> MPDFLGHAENPLREEEWARLNETVIQVARRSLVGRRILDIYGPLGAGVQTVPYDEFQGVSPGAVDIVGEQETAMVFTDARKFKTIPIIYKDFLLHWRDIEAARTHNMPLDVSAAAGAAALCAQQEDELIFYGDARLGYEGLMTANGRLTVPLGDWTSPGGGFQAIVEATRKLNEQGHFGPYAVVLSPRLYSQLHRGGEIETIRQLASDGVYQSNRLRGESGVVVSTGRENMDLAVSMDMVAAYLGASRMN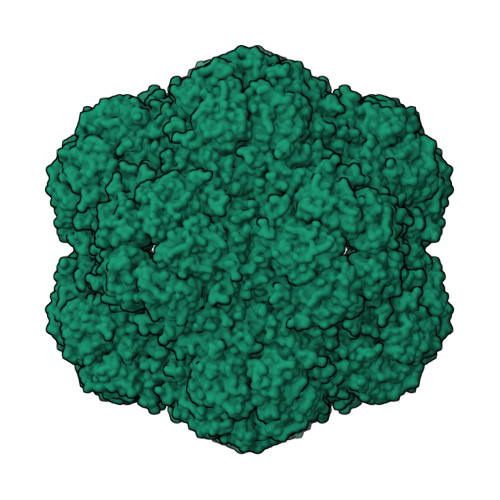HPFRVLEALLLRIKHPDAICTLEGAGATERR>[4x]MSDKTKTNEGFSRRSFIGSAAVVTAGVAGLGAIDAASATQKTNRASTVKGGFDYDVVVVGGGFAGATAARECGLQGYRTLLLEARSRLGGRTFTSRFAGQEIEFGGAWVHWLQPHVWAEMQRYGLGVVEDPLTNLDKTLIMYNDGSVESISPDEFGKNIRIAFEKLCHDAWEVFPRPHEP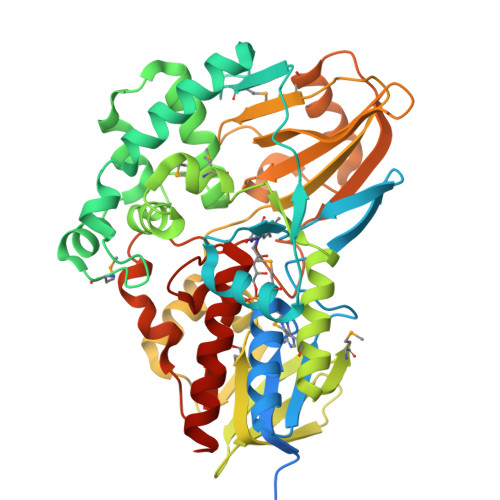MFTERARELDKSSVLDRIKTLGLSRLQQAQINSYMALYAGETTDKFGLPGVLKLFACGGWNYDAFMDTETHYRIQGGTIGLINAMLTDSGAEVRMSVPVTAVEQVNGGVKIKTDDDEIITAGVVVMTVPLNTYKHIGFTPALSKGKQRFIKEGQLSKGAKLYVHVKQNLGRVFAFADEQQPLNWVQTHDYSDELGTILSITIARKETIDVNDRDAVTREVQKMFPGVEVLGTAAYDWTADPFSLGAWAAYGVGQLSRLKDLQAAEGRILFAGAETSNGWHANIDGAVESGLRAGREVKQLLSLEHHHHHH CGS is a transferase and acts in the committed step (the fifth overall) of the biosynthesis of l-methionine. MetB is covalently linked to the cofactor pyridoxal phosphate (PLP), similar to other members of the aspartate aminotransferase (AAT-I) superfamily of enzymes. Similar to other CGS enzymes, MetB forms a homotetramer, with each individual homodimer creating two active sites. Here, we present two structures of the cystathionine γ-synthase MetB from M. ulcerans covalently linked to PLP and bound to the buffer molecule HEPES.

A second structure contains PLP as well as a highly ordered HEPES molecule in the active site acting as a pseudo-ligand. HEPES is bound in the active site with the sulfate head group pointing in towards the pocket and only 3.1 Å from the ∊-­amino group of the PLP–Lys208 moiety. The HEPES molecule is bound by a series of hydrogen bonds from the homodimer, including residues Tyr111, Asn158, Ser336, Arg368 and the PLP–Lys208 moiety of one monomer and Thr59 of the second monomer. HEPES is only found ordered in domain A; however, all the other monomers contain a well ordered sulfate at this location, suggesting that there may be a poorly ordered HEPES bound in each case. The presence of bound HEPES in the active site of MetB does not change the protein conformation locally or globally (the superposition r.m.s.d.s for MetB–PLP and MetB–PLP–HEPES were 0.134 Å for molecule A, 0.136 Å for molecule B, 0.151 Å for molecule C, 0.141 Å for molecule D and 0.15 Å overall calculated on all common Cα atoms). The only noted change is seen in a loop consisting of residues 350–362, in which the disordered loop in the MetB–PLP structure becomes partially ordered in the MetB–PLP–HEPES structure. There is no apparent conformational change observed for the PLP moiety in the presence or absence of HEPES. However, the MetB–PLP–HEPES structure suggests that the active site is likely to be blocked to binding of these molecules owing to the presence of a well ordered HEPES molecule.

>GPGSMKDDHKAQHRFAGLATRAIHSGYRPDPATGAVNAPIYASSTFAQDGVGGLRGGYEYARTGNPTRTALEAALAAVEDAAFGRAFSSGMAAADCALRAMLRPGDHVVIPDDAYGGTFRLIDKVFTGWNVEYTPVALADLDAVRAAIRPTTRLIWVETPTNPLLSIADIAGIAQLGADSSAKVLVDNTFASPALQQPLSLGADVVLHSTTKYIGGHSDVVGGALVTNDEELDQSFAFLQNGAGAVPGPFDAYLTMRGLKTLVLRMQRHSENAAAVAEFLAEHPAISTVLYPGLPSHPGHAVAARQMRGFGGMVSVRMRAGRTAAEQLCAKTNIFILAESLGSVESLIEHPSAMTHASTAGSQLEVPDDLVRLSVGIEDVADLLDDLKQALG[4x]> RLGSG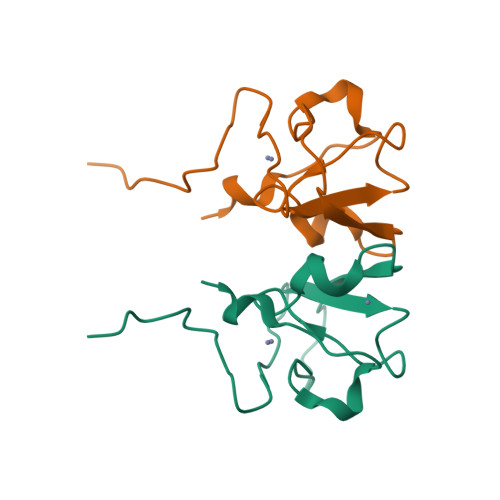DVHKHTGRNCGRKFKIGEPLYRCHECGCDDTCVLCIHCFNPKDHVNHHVCTDICTEFTSGICDCGDEEAWNSPLHCKAEEQ> VQFRGGTTAQHATFTGAAREITVDTDKNTVVVHDGATAGGFPLARHDLVKTAFIKADKSAVAFTRTGNATASIKAGTIVEVNGKLVQFTADTAITMPALTAGTDYAIYVCDDGTVRADSNFSAPTGYTSTTARKVGGFHYAPGSNAAAQAGGNTTAQINEYSLWDIKFRPAALDPRGMTLVAGAFWADIYLLGVNHLTDGTSKYNVTIADGSASPKKSTKFGGDGSAAYSDGAWYNFAEVMTHHGKRLPNYNEFQALAFGTTEATSSGGTDVPTTGVNGTGATSAWNIFTSKWGVVQASGCLWTWGNEFGGVNGASEYTANTGGRGSVYAQPAAALFGGAWNGTSLSGSRAALWYSGPSFSFAFFGARGVCDHL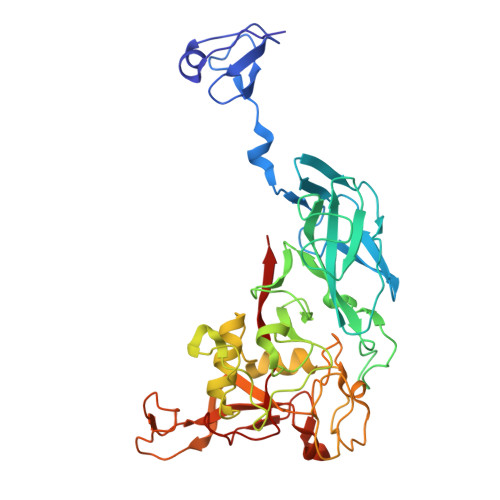IL The nuclear envelope partitions nuclear components from the cytoskeleton, thereby necessitating their mechanical coupling across the nuclear envelope to enable cytoskeletal function in the structure and positioning of nuclear contents. This is achieved by the Linker of Nucleoskeleton and Cytoskeleton (LINC) complex, which traverses the nuclear envelope and binds to cytoskeletal and nuclear structures to mediate force transduction between these partitioned components (Haque et al., 2006; Crisp et al., 2006; Lee and Burke, 2018; Meinke and Schirmer, 2015). The LINC complex is formed of SUN (Sad1 and UNC84 homology) domain and KASH (Klarsicht, ANC-1, and Syne homology) domain proteins, which interact immediately below the outer nuclear membrane, through complex formation between their C-terminal eponymous SUN and KASH domains. Thus, the LINC complex axis is established by a peri-nuclear SUN-KASH core interaction and mechanically couples the cytoskeleton and nuclear contents. We find that SUN-KASH complexes between SUN proteins and Nesprin-4, KASH5 and Nesprin-1 are 6:6 structures formed of constitutive interactions between two 3:3 complexes.

The SUN1-KASH5 crystal structure was solved at 1.54 Å resolution and revealed a similar 6:6 assembly in which opposing 3:3 complexes are held together by extensive interactions between opposing KASH5 molecules and KASH-lids. SUN1-KASH5 demonstrates the most extensive 6:6 interface in which KASH5 molecules and SUN1 KASH-lids from opposing 3:3 complexes wind around each other in a right-handed screw to create a complete circumferential interface enclosing a hollow core, similar to a β-barrel fold. KASH5 follows an almost linear path, packed between a SUN1 globular core and KASH-lids of opposing SUN1 protomers, with N-terminal 545-PPP-547 motifs of opposing molecules interacting across the interface. KASH5 and KASH4 follow similar paths, with KASH5 PPP-motif interactions and KASH4 zinc-sites located at the same positions and providing analogous interface-spanning interactions. However, an important distinction is that a torsional rotation of approximately 20° between the 3:3 complexes of SUN1-KASH5, relative to SUN1-KASH4, brings together opposing KASH-lids and enables their interaction across the interface. Thus, tip-to-tip interactions via amino acids I673 and F671 of opposing SUN1 KASH-lids contribute to the extensive 6:6 interface of SUN1-KASH5. In contrast, SUN1-KASH5 is an intermediate structure that utilises both KASH and KASH-lid mechanisms to form a fully enclosed 6:6 interface. In agreement with the equal roles of KASH domain and KASH-lid interactions at its 6:6 interface, SUN1-KASH5 exhibited intermediate phenotypes upon I673E and F671E mutation, with retention of complex formation but reduction in oligomer size to species that likely reflect partially dissociating 6:6 complexes. KASH5 functions in meiosis and is essential for fertility.

> GSGGSGGITEAQARAIVNSALKLYSQDKTGMVDFALESGGGSILSTRCSETYETKTALMSLFGIPLWYFSQSPRVVIQPDIYPGNCWAFKGSQGYLVVRLSMMIHPAAFTLEHIPKTLSPTGNISSAPKDFAVYGLENEYQEEGQLLGQFTYDQDGESLQMFQALKRPDDTAFQIVELRIFSNWGHPEYTCLYRFRVHGEPVK;> GSMTSGTSGTSGGPSPPPTWPHLQLCYLQPPPV> MQISANQYFEGIYAKYQNIEDMQATINFTLKGLKQTGVLLYKFPDKFIINLDSNNQVFVSDGEFLTVYVPSLGTSFNQQLLKGSSGGGLMKVLNSEYSVSYTNSPNLEDLDSSEPGKYIKLTFSRKLYKGAATINSFIIAFAPDGIIRRITAFPTSGGREIVIDLTAVK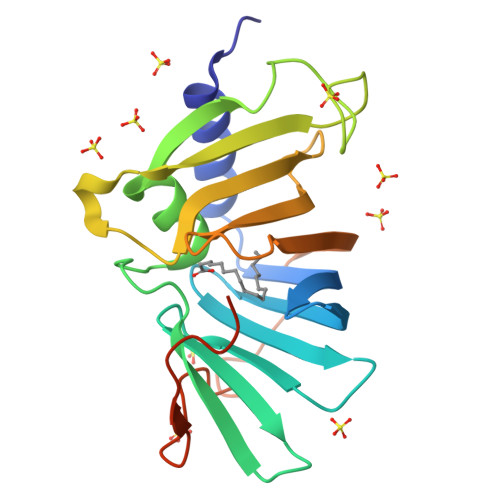FNVGILDSKFKYDPPKSSNKVDNFLYDIKKNLEHHHHHH>[2x]GREEIFQV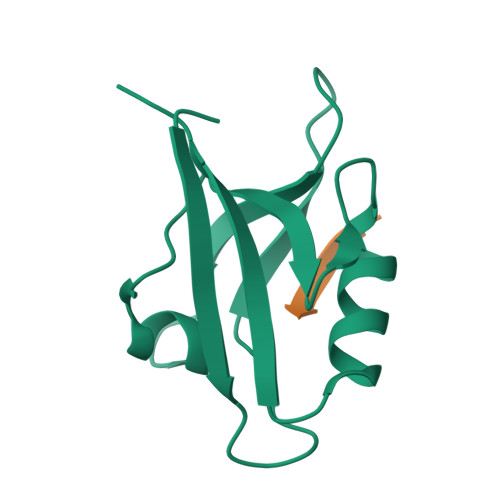ALHKRDSGEQLGIKLVRRTDEPGVFILDLLEGGLAAQDGRLSSNDRVLAINGHDLKYGTPELAAQIIQASGERVNLTIARPGKPQP;>NLNSSRVPDLLV[2x]(2~{S})-~{N}-[5-(4-bromophenyl)-1~{H}-imidazol-2-yl]-2-[4-(1-methylimidazol-4-yl)phenoxy]propanamide | C22 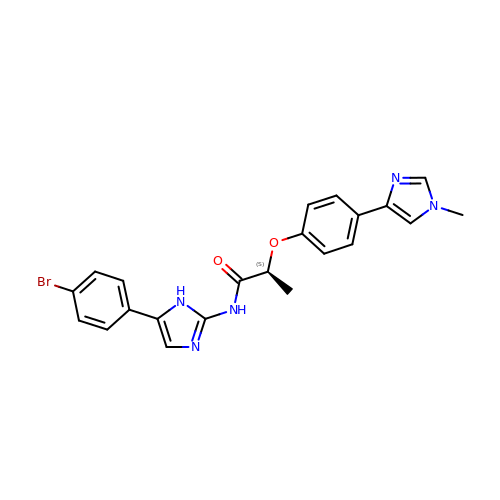H20 Br N5 O2 | NCECUTFKDWLGRR-AWEZNQCLSA-N N-[2-(morpholin-4-yl)ethyl]-6-(8-phenyl-1H-imidazo[4,5-c][1,7]naphthyridin-1-yl)-1,3-benzothiazol-2-amine | C28 H25 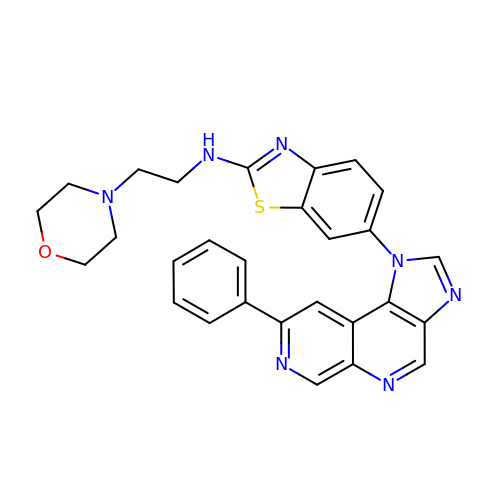N7 O S | WJOPLUBIUOVUKG-UHFFFAOYSA-N>MGSDKIHHHHHHENLYFQGMIKLIATDIDGTLVKDGSLLIDP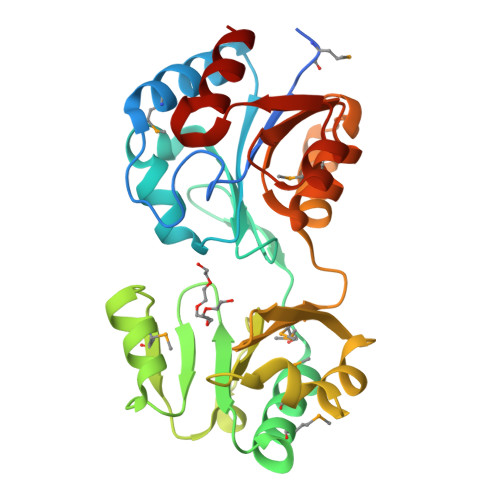EYMSVIDRLIDKGIIFVVCSGRQFSSEFKLFAPIKHKLLYITDGGTVVRTPKEILKTYPMDEDIWKGMCRMVRDELPACDYFAATPDFCFAEDGGSPIFHLLRDSYGFEMREVDDITRLDRNDIIKFTVFHPDKCEELCTPVFIPAWNKKAHLAAAGKEWVDCNAKGVSKWTALSYLIDRFDLLPDEVCCFGDNLNDIEMLQNAGISYAVSNARQEVIAAAKHTCAPYWENGVLSVLKSFL[2x]> GAMSNQHVLEEKTVAGWVAENQTALLYLMTRGQRAVRQQGESDMAGSRWYWRTTPLSTGNALLQAVDIEVSLHEDFSSVIQSRRAWFSA;> MNSAVAGHDQKLNLMQQTMSFLTHDLTQMMPRPVRGDQGQREPALLAGAGVLASESEGMRFVRGGVVNPLMRLPRSNLLTVGYRIHDGYLERLAWPLTDAAGSVKPTMQKLIPADSLRL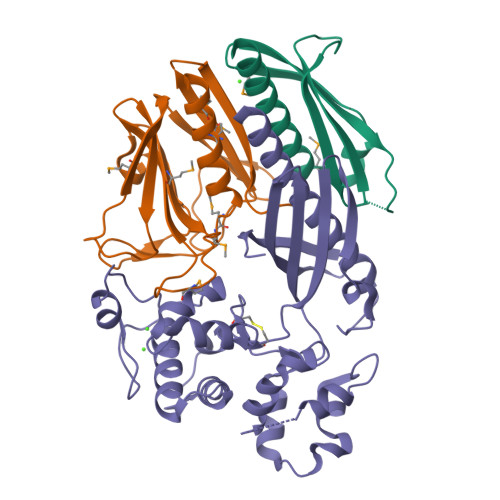QFYDGTRWQESWSSVQAIPVAVRMTLHSPQWGEIERIWLLRGPQ;> GAMGRMQQQLGRTRSQQEYQQALWYSASAESLALSALSLSLKNEKRVHLEQPWASGPRFFPLPQGQIAVTLRDAQACFNLNALAQPTTASRPLAVQQLIALISRLDVPAYRAELIAESLWEFIDEDRSVQTRLGREDSEYLARSVPFYAANQPLADISEMRVVQGMDAGLYQKLKPLVCALPMTRQQININTLDVTQSVILEALFDPWLSPVQARALLQQRPAKGWEDVDQFLAQPLLADVDERTKKQLKTVLSVDSNYFWLRSDITVNEIELTMNSLIVRMGPQHFSVLWHQTGESE>MTADELVFFVNGKKVVEKNADPETTLLVYLRRKLGLCGTKLGCGEGGCGACTVMISKYDRLQNKIVHFSVNACLAPICSLHHVAVTTVEGIGNTQKLHPVQERIARSHGSQCGFCTPGIVMSMYTLLRNQPEPTVEEIENAFQGNLCRCTGYRPILQGFRTFAKDGGCCGGSGNNPNCCMNQTKDQTVSLSPSLFNPEDFKPLDPTQEPIFPPELLRLKDTPQKKLRFEGERVTWIQASTMEELLDLKAQHPDAKLVVGNTEIGIEMKFKNMLFPLIVCPAWIPELNSVVHGPEGISFGASCPLSLVESVLAEEIAKLPEQKTEVFRGVMEQLRWFAGKQVKSVASIGGNIITASPISDLNPVFMASGAKLTLVSRGTRRTVRMDHTFFPGYRKTLLRPEEILLSIEIPYSKEGEFFSAFKQASRREDDIAKVTSGMRVLFKPGTIEVQELSLCFGGMADRTISALKTTPKQLSKSWNEELLQSVCAGLAEELQLAPDAPGGMVEFRRTLTLSFFFKFYLTVLQKLGRADLEDMCGKLDPTFASATLLFQKDPPANVQLFQEVPKDQSEEDMVGRPLPHLAANMQASGEAVYCDDIPRYENELSLRLVTSTRAHAKITSIDTSEAKKVPGFVCFLTAEDVPNSNATGLFNDETVFAKDEVTCVGHIIGAVVADTPEHAQRAARGVKITYEDLPAIITIQDAINNNSFYGSEIKIEKGDLKKGFSEADNVVSGELYIGGQEHFYLETNCTIAVPKGEAGEMELFVSTQNTMKTQSFVAKMLGVPDNRIVVRVKRMGGGFGGKETRSTVVSTALALAAHKTG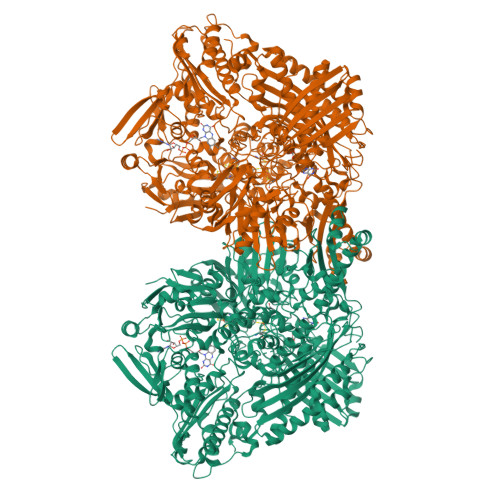RPVRCMLDRDEDMLITGGRHPFLAKYKVGFMKTGTVVALEVAHFSNGGNTEDLSRSIMERALFHMDNAYKIPNIRGTGRICKTNLPSNTAFRGFGGPQGMLIAEYWMSEVAITCGLPAEEVRRKNMYKEGDLTHFNQKLEGFTLPRCWDECIASSQYLARKREVEKFNRENCWKKRGLCIIPTKFGISFTLPFLNQGGALVHVYTDGSVLLTHGGTEMGQGLHTKMVQVASRALKIPTSKIHISETSTNTVPNTSPTAASASADLNGQGVYEACQTILKRLEPFKKKKPTGPWEAWVMDAYTSAVSLSATGFYKTPNLGYSFETNSGNPFHYFSYGVACSEVEIDCLTGDHKNLRTDIVMDVGSSLNPAIDIGQVEGAFVQGLGLFTMEELHYSPEGSLHTRGPSTYKIPAFGSIPIEFRVSLLRDCPNKRAIYASKAVGEPPLFLASSIFFAIKDAIRAARAQHGDNAKQLFQLDSPATPEKIRNACVDQFTTLCVTGVPENCKSWSVRI[2x]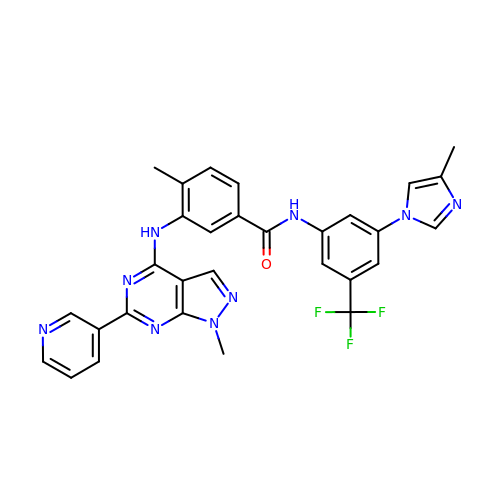4-methyl-~{N}-[3-(4-methylimidazol-1-yl)-5-(trifluoromethyl)phenyl]-3-[(1-methyl-6-pyridin-3-yl-pyrazolo[3,4-d]pyrimidin-4-yl)amino]benzamide | C30 H24 F3 N9 O | PURQMMYVBMISCI-UHFFFAOYSA-N>GTHMNK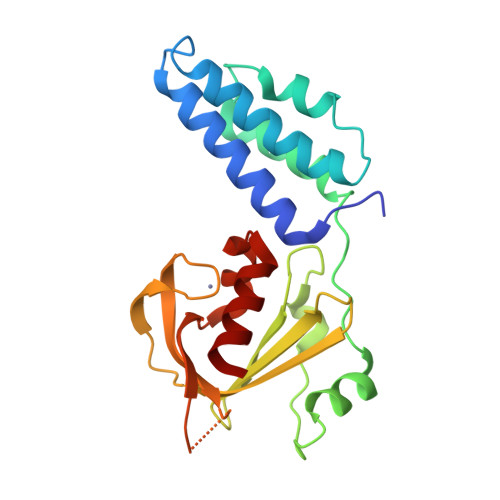IEVYKFVKVKQLVYQLIKLYRTNDMNSHKTQKDFLLNEINDIFKEKDIDISDFITSIDDVKLTKKKAEHLLNELKVYIQDFEIPSSSQLEKIFRKVKKLKRPDINLIDTKEISYLGWNDNSSNRKYIVYKNLDDKFEGIYGEISPNKVKGFCKICNQESDTSLFLNKTKHNKSSGTYTKKGDYICYDSFKCNQNLDDINNLYEFIVKIK[2x]>[2x]MQNYNAKSIEVLTGLDPVKKRPGMYTNIENPNHLIQEIIDNSVDEVLAGFASKINITLYEDNSIEVADDGRGMPVDIHPEHKMSG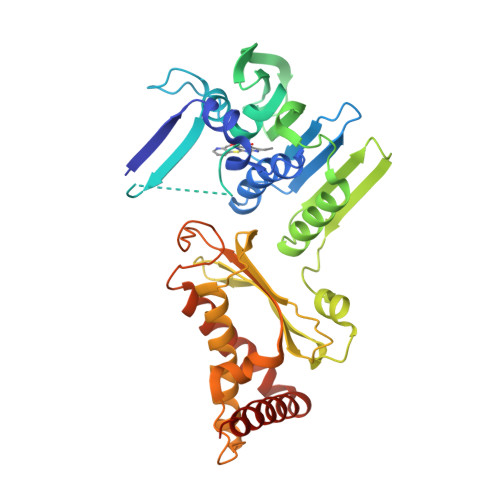IELIMTKLHSGGKFSNKNYTHSGGLHGVGVSVVNALSTRLEAEIKRDGNVYHIVFEDGFKTKDLEIIDNVGKKNTGTKIRFWPNKKYFDDIKVNFKALKNLLEAKAILCKALTIKYSNEIKKEKLTWHFETGLKGYLDHKLEAETLPAEPFIIDNFSNGDSYLDAVFCWCEDPSESIKNSYVNLIPTPQDGTHVTGLKNGIYDAIKAYIEKNSLSVKNIKITANDSFAQLNYVISVKITNPQFAGQTKEKLSNKDVTNFVATAVKDLLTIWLNQNPDEARQIVENISKVAQKRINADLEHHHHHH> MSGAVYFLLLDLRAEVDEEIAWARRLGLDDLVAALEAVRALIEGALATLESADFDYLEFTQRLADALSSLVRVYDDLIARLEEQPATTLRRAYRILLEYRRKEVRELLEAVQELRDVLETLERLSRRLGRPDFAGWLVSFVLDHYGELVAPDILTNPAKGFRALAHLLRAFLYVLLALKLRSPDEELREEARRAVAFLYGEEFVKAHSDEELAELLLERAREAILEAARYNSALREEFDAAGGPEGREAWLERQLLRLRGLVERFLELWENSELRAGPDGELVAVPGVKGLEIIKKLLEEGKGVNLALWTLGRLLRALDLSPEARAAYEAALEALRRARLQLQYVQSERYEGSDRERAEAIRAAFETIRAAAETIRAVIEADTSLPAELKAAYIEVIYAYLLQVAREVRDALWRLAEEILPEYIEKFFKGSEEEQRLTLYELLRALGEDYFFLDLEKEGYSEEELRELFRNAKLEVINADESGKIKLYNLILDAKKLNRKVLIKITLTELSEGSYIITIEVFKSPDAEIPEYEIRVAAVGATSEEILKYLEELKEKAKEGELIRELLLLYVDRQIAELEEKVANADKIDPVVARLAIEEARARGEELTEADVIE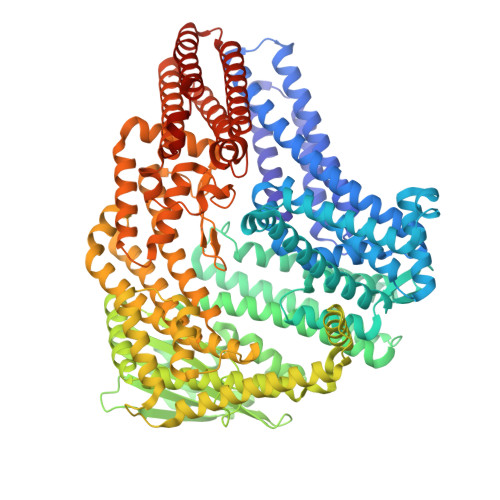GTRAGYQAALDVLRRIKAELEKEKSPENPFYQFYDKLTEKLKEKGFVSEEEAFEIARETFGFPADLPPLAAAALRDFASTVLTILEIFKTAEDFSKWYKENKEKLIELAGLSEEELDKIVRKTLTLLLEALARSVFGSKLGRELLNEALGTFIKELLESFFRTHYGLTRGDAVIDFDAKTGILSLRFTPRAYARIRVKEYRDPSLGEKFDNLLDVLSSNPSLKGQVDRLRVSYAFGTPVGTTPALRDATAEDLETDPRLKRHRDFIEEVENLYAELLIRLEEALKDEPETVEILTEIIGRHLKEVIHDPDVINALLDRRDLSPEEFAARARAVLDEIIAEEKKLQEKLLEAVEDNPEAKKIVEEIFPKIIATIERYREWPERELAGLPLGGSHHHHHH>[2x]MGLEPEFSGNGDVQIPNGDFETGNLSGWTGWGGTIRDITATNAYEGGFAG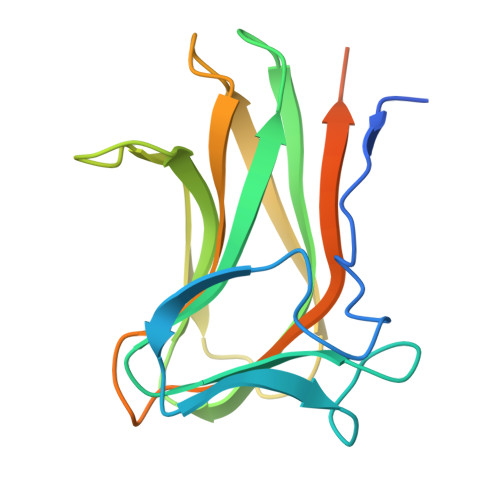HIKGAGAHEKEVSLRPNTQYVLSAYIKVASGNIIFGIKENTANAQAIASTTLNNTEYQKVELSFTTGSETNLKLFLFAQQATDEGFGDNFEITSLGGDNRPTKPAIFTEEFLEHHHHHH>[2x]MKALTARQQEVFDLIRDHISQTGMPPTRAEIAQRLGFRSPNAAEEHLKALARKGVIEIVSGASRGIRLLQEEEEGLPLV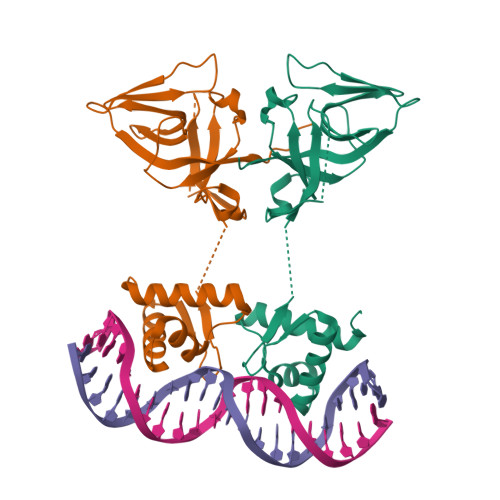GRVAAGEPLLAQQHIEGHYQVDPSLFKPNADFLLRVSGMSMKDIGIMDGDLLAVHKTQDVRNGQVVVARIDDEVTVARLKKQGNKVELLPENSEFKPIVVDLRQQSFTIEGLAVGVIRNGDWL> NKICQFKLVLLG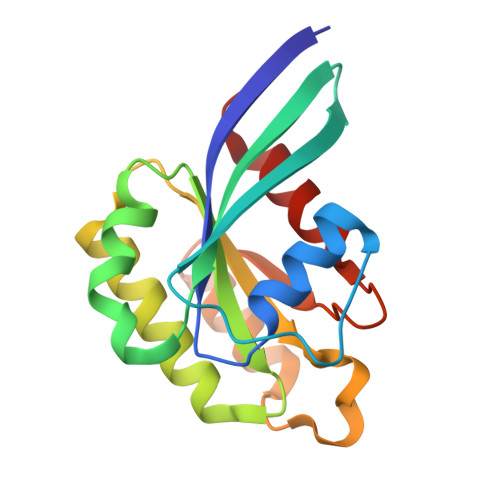ESAVGKSSLVLRFVKGQFHEFQESTIGAAFLTQTVCLDDTTVKFEIWDTAGLERYHSLAPMYYRGAQAAIVVYDITNEESFARAKNWVKELQRQASPNIVIALSGNKADLANKRAVDFQEAQSYADDNSLLFMETSAKTSMNVNEIFMAIAKKLPK>MVKIVTVKTQAYQDQKPGTSGLRKRVKVFQSSANYAENFIQSIISTVEPAQRQEATLVVGGDGRFYMKEAIQLIARIAAANGIGRLVIGQNGILSTPAVSCIIRKIKAIGGIILTASHNPGGPNGDFGIKFNISNGGPAPEAITDKIFQISKTIEEYAVCPDLKVDLGVLGKQQFDLENKFKPFTVEIVDSVEAYATMLRSIFDFSALKELLSGPNRLKIRIDAMHGVVGPYVKKILCEELGAPANSAVNCVPLEDFGGHHPDPNLTYAADLVETMKSGEHDFGAAFDGDRDRNMILGKHGFFVNPSDSVAVIAANIFSIPYFQQTGVRGFARSMPTSGALDRVASATKIALYETPTGWKFFGNLMDASKLSLCGEESFGTGSDHIREKDGLWAVLAWLSILATRKQSVEDILKDHWQKYGRNFFTRYDYEEVEAEGANKMMKDLEALMFDRSFVGKQFSANDKVYTVEKADNFEYSDPVDGSISRNQGLRLIFTDGSRIVFRLSGTGSAGATIRLYIDSYEKDVAKINQDPQVMLAP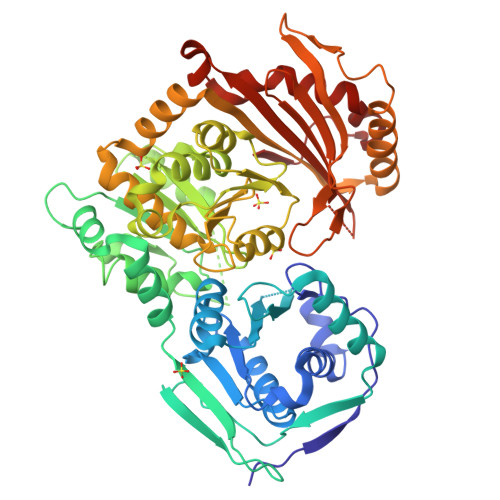LISIALKVSQLQERTGRTAPTVIT[2x]> MSSQIRQNYSTEVEAAVNRLVNLYLRASYTYLSLGFYFDRDDVALEGVCHFFRELAEEKREGAERLLKMQNQRGGRALFQDLQKPSQDEWGTTPDAMKAAIVLEKSLNQALLDLHALGSAQADPHLCDFLESHFLDEEVKLIKKMGDHLTNIQR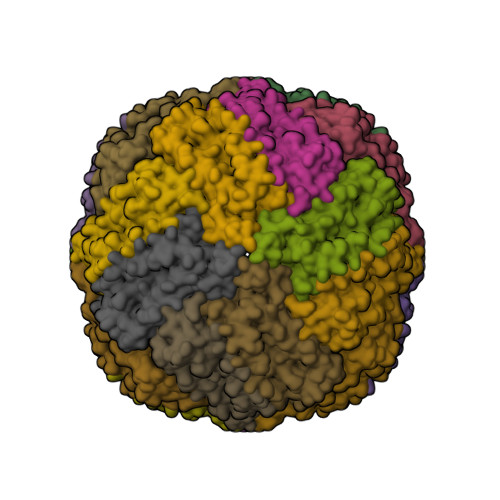LVGSQAGLGEYLFERLTLKHD>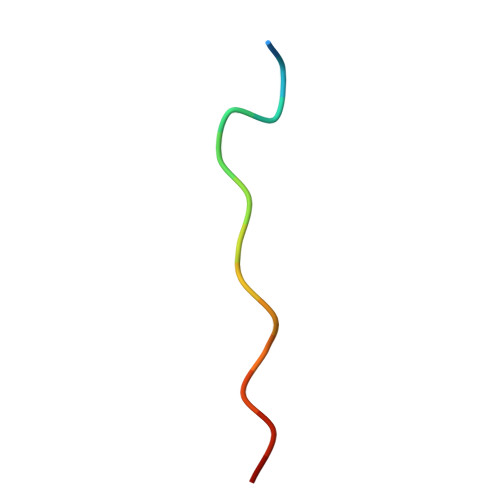 KNMTPYRSPPPYVPP> GMSFLFSSRSSKTFKPKKNIPEGSHQYELLKHAEATLGSGNLRQAVMLPEGEDLNEWIAVNTVDFFNQINMLYGTITEFCTEASCPVMSAGPRYEYHWADGTNIKKPIKCSAPKYIDYLMTWVQDQLDDETLFPSKIGVPFPKNFMSVAKTILKRLFRVYAHIYHQHFDSVMQLQEEAHLNTSFKHFIFFVQEFNLIDRRELAPLQELIEKLGSKDR;> MHHHHHHGSGDKEKKQITTSPITVRKNKKDEERRESRIQSY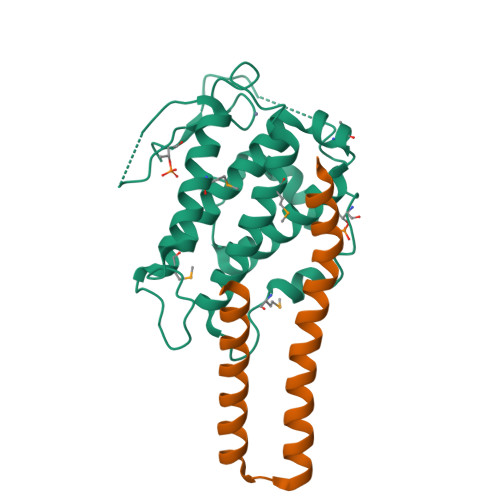SPQAFKFFMEQHVENVLKSHQQRLHRKKQLENEMMRVGLSQDAQDQMRKMLCQKESNYIRLKRAKMDKSM>[4x]SNAMSEFIMNNLEQTARRWLEERGVTVEKIAELVYYLQSKYHPDLTME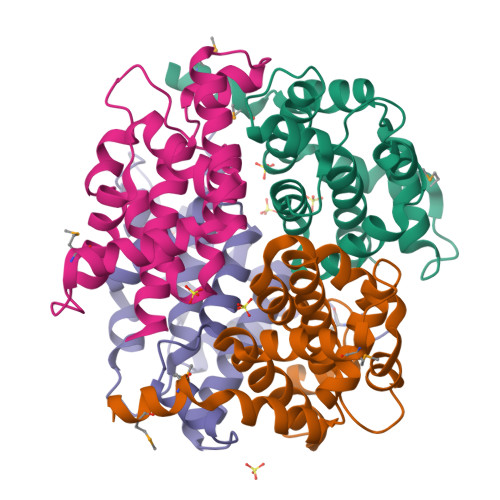ECIENVNRVISKREVQNAILTGIQLDKLAEDGRLDEPLQSIIRRDEGLYGVDEILALSIVNVYGSIGFTNYGYIDKQKPGILQYLNDKSTGKCNTFLDDIVGAIAAAASSRLAHRAANAE> MRVLGIETSCDETAVAVLDDGKNVVVNFTVSQIEVHQKFGGVVPEVAARHHLKNLPILLKKAFEKVPPETVDVVAATYGPGLIGALLVGLSAAKGLAISLEKPFVGVNHVEAHVQAVFLANPDLKPPLVVLMVSGGHTQLMKVDEDYSMEVLGETLDDSAGEAFDKVARLLGLGYPGGPVIDRVAKKGDPEKYSFPRPMLDDDSYNFSFAGLKTSVLY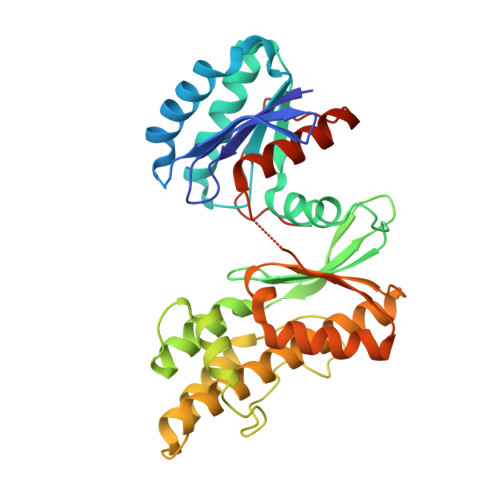FLQREKGYKVEDVAASFQKAVVDILVEKTFRLARNLGIRKIAFVGGVAANSMLREEVRKRAERWNYEVFFPPLELCTDNALMVAKAGYEKAKRGMFSPLSLNADPNLNV> MHHHHHHSSGKWGRVLAILKAFEEDCATPISKLRQVADAMTVEMHAGLASDGGSKLKMLISYVDNLPSGDEKGLFYALDLGGTNFRVMRVLLGGKQERVVKQEFEEVSIPPHLMTGGSDELFNFIAEALAKFVATECEDFHLPEGRQRELGFTFSFPVKQTSLSSGSLIKWTKGFSIEEAVGQDVVGALNKALERVGLDMRIAALVNDTVGTLAGGRYYNPDVVAAVILGTGTNAAYVERATAIPKWHGLLPKSGEMVINMEWGNFRSSHLPLTEFDHTLDFESLNPGEQILEKIISGMYLGEILRRVLLKMAEDAAFFGDTVPSKLRIPFIIRTPHMSAMHNDTSPDLKIVGSKIKDILEVPTTSLKMRKVVISLCNIIATRGARLSAAGIYGILKKLGRDTTKDEEVQKSVIAMDGGLFEHYTQFSECMESSLKELLGDEASGSVE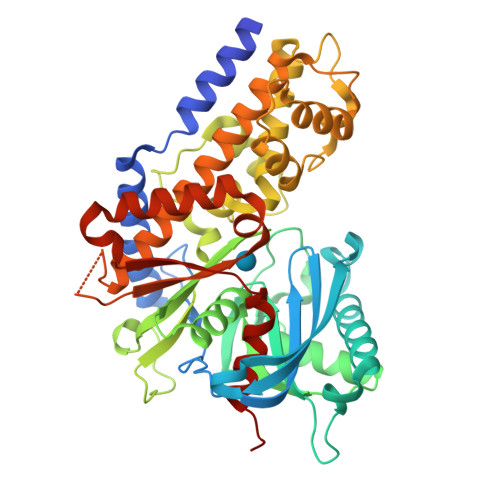VTHSNDGSGIGAALLAASHSLYLEDS> MGSNQSSSTSTKKLKAGNFDVAYQNPDKAIKGGNLKVAYQSDSPMKAQWLSGLSNDATFATMSGPGGGQDGLFFTDSGFKFI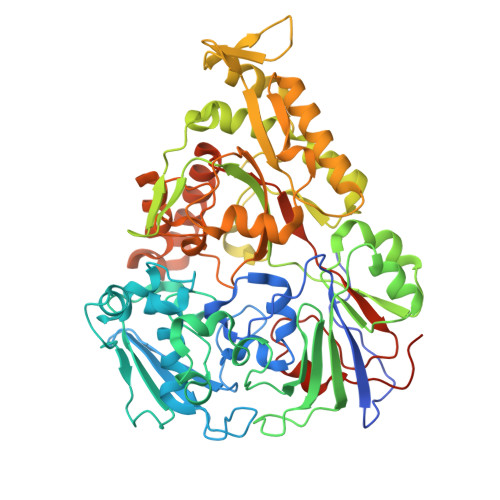KGGAADVALDKESKTATITLRKDLKWSDGSEVTAKDYEFTYETIANPAYGSDRWTDSLANIVGLSDYHTGKAKTISGITFPDGENGKVIKVQFKEMKPGMTQSGNGYFLETVAPYQYLKDVAPKDLASSPKTTTKPLVTGPFKPENVVAGESIKYVPNPYYWGEKPKLNSITYEVVSTAKSVAALSSSKYDIINGMVSSQYKQVKNLKGYKVLGQQAMYISLMYYNLGHYDAKNSINVQDRKTPLQDQNVRQAIGYARNVAEVDNKFSNGLSTPANSLIPPIFKQFTSSSVKGYEKQDLDKANKLLDEDGWKLNKSTGYREKDGKELSLVYAARVGDANAETIAQNYIQQWKKIGVKVSLYNGKLMEFNSWVDHMTTPPGANDWDITDGSWSLASEPSQQDLFSAAAPYNFGHFNDSEITKDLNDIDSAKSENPTYRKAAFVKYQEDMNKKAYVIPTNFMLNYTPVNKRVVGMTLDYGAMNTWSEIGVSSAKLATKGSIEGRHHHHHH> MNTISVKAMSKSSDTTEITSQSTTKLRNVMYYGDWSIWGGQGNFYPKDIPADKLTHLNFAFMDFNSSGELIYCDKDAAIGHPLGNLGVTYGDVNGGILNAFQVLKSENPNLKIGVSLGGWSKSGDFSTIAATPSIRAKFVENVMKFIKYTNMDFVDIDWEYPGDYREPDKTDNINDEGTPNASAGDKENYILLLQDLKEALNKQGKELGKVYELSVALPAGVSKIEKGIDVDKLFNIVDFANIMTYDMAGAWSTTSGHQTALYTNPNAPEEYKGLSVDESVKYYISQGAEREKIVVGAAYYTRGWEQVSDKGTDPNNPGLFGEAAVVNKDADLSPTPGALNEAPMKNGEGGRAGGVWGYNALDKLKSKYTGLKEYWDDSAKAPYLYNSETGAFFTYDNIRSIQEKAKYVKENNLGGIIGWMASQDATTNSTKRDELTTATKESLFGKEDLPKYEIKYTENDITCTVTPVKQSWGSGGVLKMSITNNEKLDESGEVLSTVETSAKTVKNMKVYIKTDGIAITGSQYPAGPVTKEGDYYVIDFGKISDGKLMKAGITFTFDLNLDKAIEDTNNIISIEVSQRMYQTSPEFNRQTIWENTNSPRNKGELEGKPIPNPLLGLDSTRTGHHHHHH

C. perfringens type G, the causative agent of necrotic enteritis in broilers, produces two glycosyl hydrolase family 18 chitinases, ChiA and ChiB, which display distinct substrate preferences. Whereas ChiB preferentially processes linear substrates such as chitin, ChiA prefers larger and more branched substrates, such as carbohydrates presented by the chicken intestinal mucus. Here, we show via crystal structures of ChiA and ChiB in the apo and ligand-bound forms that the two enzymes display structural features that explain their substrate preferences providing a structural blueprint for further interrogation of their function and inhibition. We succeeded in obtaining several crystal structures of recombinant ChiA and ChiB in apo (unbound) and ligand-bound forms to resolutions between 1.30 Å and 1.85 Å. Both ChiA and ChiB encode for an N-terminal glycosyl hydrolase family 18 (GH18) Trios-phosphate Isomerase (TIM) barrel followed by a C-terminal putative carbohydrate binding domain (CBD).

When comparing the overall structures of the chitinases, the unexpected location of the ChiB CBD becomes apparent. As compared to ChiA and the Chromobacterium violaceum chitinase, the CBD of ChiB is located on the opposite side of the TIM barrel. This CBD-location of ChiB is similar to the one occupied by the Serratia marcescens ChiA CBD. The cleft of ChiB is covered by a loop of the TIM barrel leaving only the sides open to the solvent. As in ChiA, the sizeable substrate binding pocket of Apo ChiB contained a PIPES buffer molecule originating from the crystallization condition. The makeup of the binding pocket is conserved, except for the longer loop closing of the cleft and the entry of the cleft near the ChiB CBD. Neither differences should prohibit the binding of a linear chitin oligosaccharide. The active site motif is trapped in the resting conformation with a low-barrier hydrogen bond between D156 and D158. Indeed, ChiB was predicted to have a typical substrate-binding cleft of subfamily A chitinases, suggested to facilitate the hydrolysis of oligosaccharide dimers from the polysaccharide chains such as chitin, by “sliding” the substrate through the substrate-binding cleft. Overall, ChiB displays the hallmarks of a chitinase processing chitin from its reducing end towards the non-reducing end.> GHMVTRIENLENAKKLWDNANSMLEKGNISGYLKAANELHKFMKEKNLKEDDLRPELSDKTISPKGYAILQSLWGAASDYSRAAATLTESTVEPGLVSAVNKMSAFF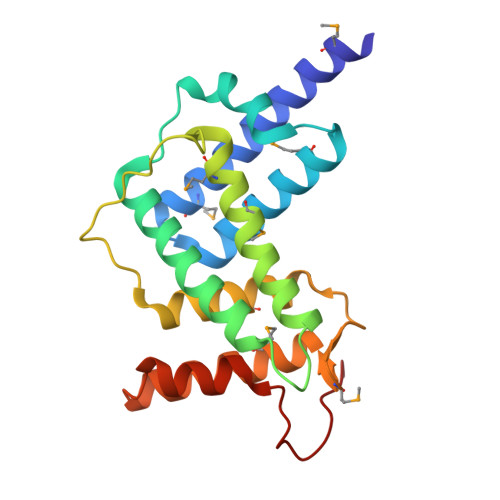MDCKLSPNERATPDPDFKVGKSKILVGIMQFIKDVADPTSKIWMHNTKALMNHKIAAIQKLERSNNVNDETLESVLSSKGENLSEYLSYK> FADDHAMSPDM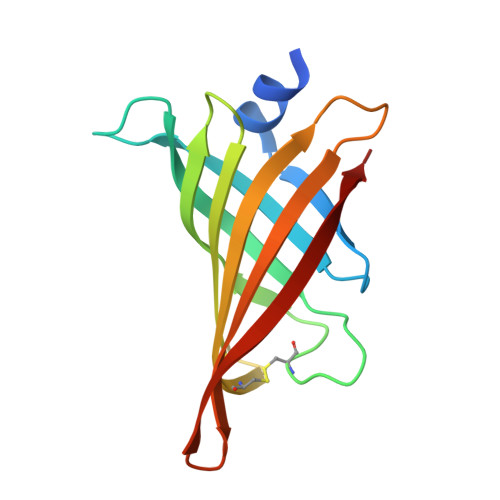KLLAGASNWVNQSGSVAQFVFTPSPTQPQTYEVSGNYINNAQGTGCKGTPYPLSGAYYSGNQIISFSVVWSNASANCQSATGWTGYFDFSGSQAVLKTDWNLAFYSGSTPAIQQGQDDFMQSV>MSRKPLIAGNWKMNLNHYEAIALVQKIAFSLPDKYYDRVDVAVIPPFTDLRSVQTLVDGDKLRLTYGAQDLSPHDSGAYTGDVSGAFLAKLGCSYVVVGHSERRTYHNEDDALVAAKAATALKHGLTPIVCIGEHLDVREAGNHVAHNIEQLRGSLAGLLAEQIGSVVIAYEPVWAIGTGRVASAADAQEVCAAIRKELASLASPRIADTVRVLYGGSVNAKNVGDIVAQDDVDGGLVGGAS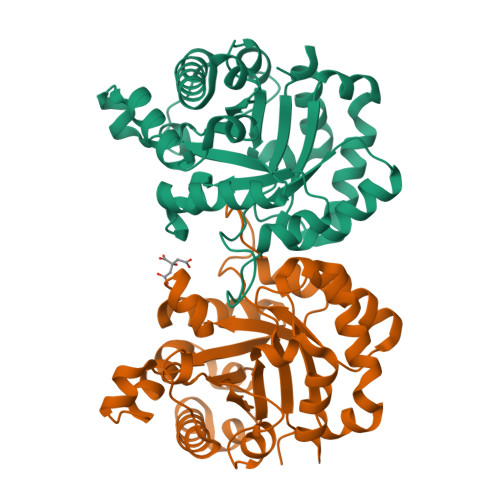LDGEHFATLAAIAAGGPLPHHHHHH[2x]> GDYCGQWDWAKSTNYIVYNNLWNKNAAASGSQCTGVDKISGSTIAWHTSYTWTGGAATEVKSYSNAALVFSKKQIKNIKSIPTKMKYSYSHSSGTFVADVSYDLFTSSTASGSNEYEIMIWLAAYGGAGPISSTGKAIATVTIGSNSFKLYK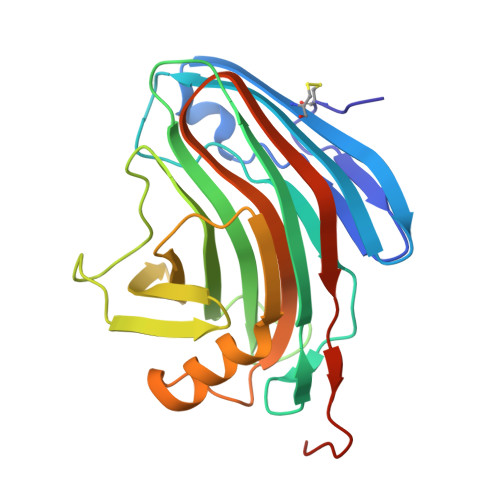GPNGSTTVFSFVATKTITNFSADLQKFLSYLTKNQGLPSSQYLITLEAGTEPFVGTNAKMTVSSFSAAVNEQKLISEEDLHHHHHH>[2x]MSGSMKEEIKRLAEELKE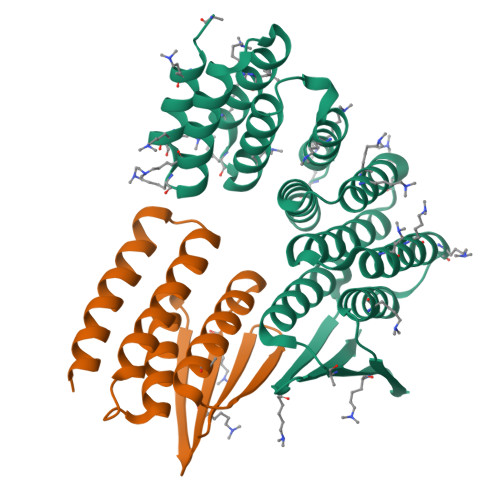KTKNEEIKRLAEEAAELAERSDDPEVLEVVKKALEEALKSKNEEKIELLLLVAVLVAEAGSVDAVEEKLEIALLALKLAEESKDPRIIRGALRAAIAALRSDDPLALKTVKEALERARASKDERLIRAILAAAYAFALLAVAGASAERLKEAEAIVKELIAAAEKGASPQELVLLVIEMMVKGMGVTMETHRSGNEVKVVIKGLHESQQEVLLEAVLFAAELMGVRVRIRFKGDTVTIVVREGSG;>[2x]MSGEEAVRRRFEELLREALAFRERTGGRRETLEHAVRLARELAEFAASHPEFNRQEAVLLAIELMVRAMGVTMETHRSGNEVKVVIKGLNIDEQVALYRAVRETSKIMGVETEIEVEGDTQTIVVREGSG>[2x]MTIPTLYMNDGMNAQSSQALHIQTYCNSVRQQIPVDFGRFPNLRESERQINTGLGAARQHAEHYLKDIQPLIIRNVTNIQDYFETQNLISTVMPSGATKEQWLSALGMVSDKAKEYQEVSANTRRTIGSLNDKLIIDSNNYQLIVVNLNNVVNGNNGVLEQLNRDIDGINAAIDGAIAGIVVGGLLVIGGAIVTAIGAVAGLVTAGTSTPVVMGGIAMMTAGAGGVIGGAIVLDKSLSAREKLYRDRSQLNSEVLVASQIGSGYRGLQTQAQSAVTAATQMNNAWDSLTSELETLNANLRKGIIDDSFLRQLFLTASQTSVTKVLDGTKIIKQQMAGVVVREVPANQSIADFVKRLAALEHHHHHH

Tripartite α-PFTs are members of the ClyA α-PFT family. Proteins in this family undergo a large scale conformational change from a compact soluble structure, where the hydrophobic residues are hidden often within a β-tongue motif, to an extended pore structure with the hydrophobic residues exposed in two extended α-helices which insert into the cell membrane. Here we show that S. marcescens has a tripartite haemolytic α-PFT (SmhABC), and propose a mechanism of pore assembly. We present the structures of the soluble A component (SmhA), as well as the soluble and pore conformations of the B component (SmhB).

As expected, soluble SmhB folds into the family observed β-tongue structure, with a five-helix bundle tail (α1, α2, α3, α6, α7), and a head domain containing three α-helices (α4, α5, α8) alongside a four-strand β-sheet (β1, β2, β3, β4), which includes the β-tongue motif (β1 and β2). The head domain of SmhB is largely hydrophobic. This is particularly evident in the β-tongue and helices α4 and α5, which together constitute the predicted hydrophobic transmembrane region (G175—L233). The B and C components interact at a binding interface located around residues 95–123 of SmhB, this could break latches 1 and 2 on the B component, releasing the β-tongue, C-terminus, and N-terminus to initiate the transformation into the B component pore conformation. The release of the C-terminus from the β-tongue agrees with the observation that the start of the conformational transition in NheA occurs at the C-terminus. This is further evidenced in the structure of a second crystal form of SmhB, where comparison of the B-factors for the two chains in the asymmetric unit revealed high flexibility at residues 85–124 and residues 280–320, corresponding to the proposed binding sites to SmhC and SmhA, indicating that movement in these binding regions can occur to facilitate complex formation.>[4x]MGHHHHHHGLSSSPSEILQELGKGSTHPQPGVSPPAAPAAPGPKDGPGETDAFGNSEGKELVASGENKIKQGLLPSLEDLLFYTIAEGQEKIPVHKFITALKSTGLRTSDPRLKECMDMLRLTLQTTSDGVMLDKDLFKKCVQSNIV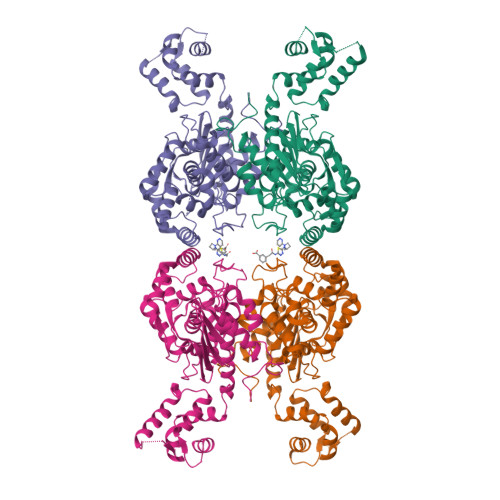LLTQAFRRKFVIPDFMSFTSHIDELYESAKKQSGGKVADYIPQLAKFSPDLWGVSVCTVDGQRHSTGDTKVPFCLQSCVKPLKYAIAVNDLGTEYVHRYVGKEPSGLRFNKLFLNEDDKPHNPMVNAGAIVVTSLIKQGVNNAEKFDYVMQFLNKMAGNEYVGFSNATFQSERESGDRNFAIGYYLKEKKCFPEGTDMVGILDFYFQLCSIEVTCESASVMAATLANGGFCPITGERVLSPEAVRNTLSLMHSCGMYDFSGQFAFHVGLPAKSGVAGGILLVVPNVMGMMCWSPPLDKMGNSVKGIHFCHDLVSLCNFHNYDNLRHFAKKLDPRREGGDQRHSFGPLDYESLQQELALKETVWKKVSPESNEDISTTVVYRMESLG pyrrolo[1,2-a]quinoxalin-4(5H)-one | C11 H8 N2 O | 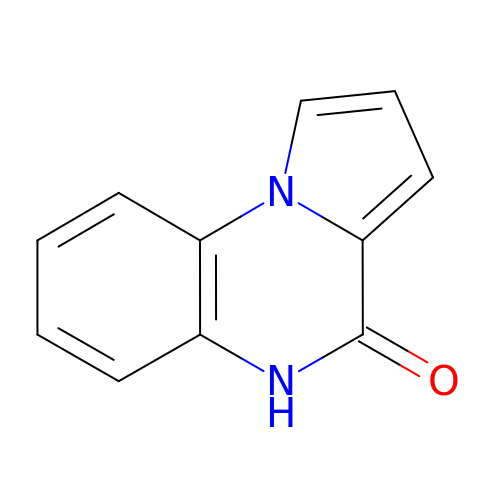LINHQLFBBDHSEJ-UHFFFAOYSA-N Two Cas12i (Cas12i1 and Cas12i2) proteins have crRNA-guided dsDNA cleavage activity. In addition to the double-strand DNA (dsDNA) cleavage activity, Cas12i2 cleaves ssDNA in trans upon crRNA forming heteroduplex with the complementary ssDNA, as well as processes the pre-crRNA to form the mature crRNA. The Cas12i2 consists of the recognition (REC) and nuclease (NUC) lobes connected by the wedge (WED) domain. The RuvC domain is the sole DNase catalytic domain in Cas12i2, with catalytic residues Asp599, Glu833, and Asp1019 lining the active pocket.

In the DNA-bound Cas12i2 ternary complexes, a 5-nt ssDNA, which was probably introduced with the target DNA, is observed in the RuvC catalytic pocket. In the Cas12i2E833A ternary complex, Mg2+A is seen, but Mg2+B is missing due to the Glu833 mutation. The Mg2+A cation is located in a similar position to Mg2+A in the Cas12i2wt complex. However, unlike the Cas12i2wt Mg2+A, the Cas12i2E833A Mg2+A coordinates an extra water and not the scissile phosphate. In the Cas12i2E833A complex, the nucleophile water is no longer positioned in-line with the phosphate and the leaving group. Superposition of the Cas12i2wt and Cas12i2E833A complexes shows that the scissile phosphate in the Cas12i2E833A complex shifts ~1.3 Å away from Mg2+A, preventing their coordination. Thus, the binding of two Mg2+ ions is essential for the proper conformation of ssDNA substrate.

> SMSSAIKSYKSVLRPNERKNQLLKSTIQCLEDGSAFFFKMLQGLFGGITPEIVRFSTEQEKQQQDIALWCAVNWFRPVSQDSLTHTIASDNLVEKFEEYYGGTASDAIKQYFSASIGESYYWNDCRQQYYDLCRELGVEVSDLTHDLEILCREKCLAVATESNQNNSIISVLFGTGEKEDRSVKLRITKKILEAISNLKEIPKNVAPIQEIILNVAKATKETFRQVYAGNLGAPSTLEKFIAKDGQKEFDLKKLQTDLKKVIRGKSKERDWCCQEELRSYVEQNTIQYDLWAWGEMFNKAHTALKIKSTRNYNFAKQRLEQFKEIQSLNNLLVVKKLNDFFDSEFFSGEETYTICVHHLGGKDLSKLYKAWEDDPADPENAIVVLCDDLKNNFKKEPIRNILRYIFTIRQECSAQDILAAAKYNQQLDRYKSQKANPSVLGNQGFTWTNAVILPEKAQRNDRPNSLDLRIWLYLKLRHPDGRWKKHHIPFYDTRFFQEIYAAGNSPVDTCQFRTPRFGYHLPKLTDQTAIRVNKKHVKAAKTEARIRLAIQQGTLPVSNLKITEISATINSKGQVRIPVKFDVGRQKGTLQIGDRFCGYDQNQTASHAYSLWEVVKEGQYHKELGCFVRFISSGDIVSITENRGNQFDQLSYEGLAYPQYADWRKKASKFVSLWQITKKNKKKEIVTVEAKEKFDAICKYQPRLYKFNKEYAYLLRDIVRGKSLVELQQIRQEIFRFIEQDCGVTRLGSLSLSTLETVKAVKGIIYSYFSTALNASKNNPISDEQRKEFDPELFALLEKLELIRTRKKKQKVERIANSLIQTCLENNIKFIRGAGDLSTTNNATKKKANSRSMDWLARGVFNKIRQLAPMHNITLFGCGSLYTSHQDPLVHRNPDKAMKCRWAAIPVKDIGDWVLRKLSQNLRAKNIGTGEYYHQGVKEFLSHYELQDLEEELLKWRSDRKSNIPCWVLQNRLAEKLGNKEAVVYIPVRGGRIYFATHKVATGAVSIVFDQKQVWVCNADHVAAANIALTVKGIGEQSSDEENPDGSRIKLQLTS methyl 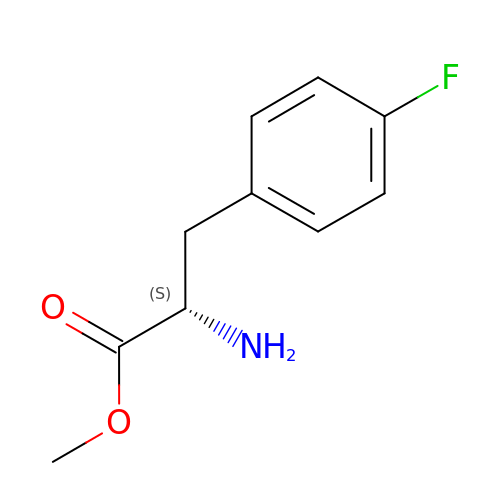4-fluoro-L-phenylalaninate | C10 H12 F N O2 | NCSHKOSBEYDZFY-VIFPVBQESA-N>EAGGVFKLIANDGKADRMIMANDLLNDRIKSIMCLRAKQGFSDPTPTLVDIERTHILLINSHYKPFAAMGYEYQKTRPNTGNPTYNSTIQFSIPQFGDFFSDMVVHVQLAATSASAGTVPALPAFIGADDQVLTSTSVVSATENTTSGVYTLYTQSYVNQQGTTQTVAAAATNFVRYCEYPGLRLFKRVKFEVNGNPLDEYTALAAIMYNKFHVPDFKLTGWKRLIGQEVPVEAASNLVNIASTTPWGSPIVALSDVNGTAVTGSPVNA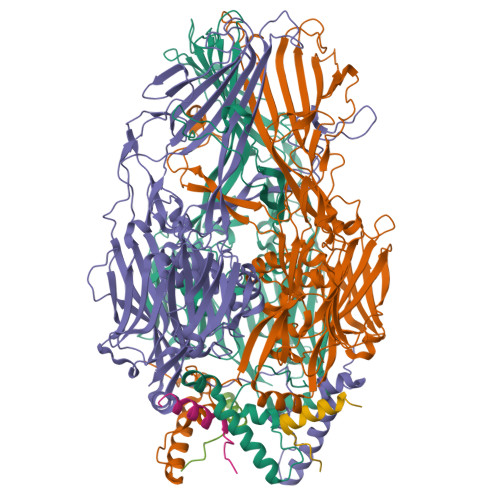AITARKLTQVVFGAQTPKATQEQLNMFVPLLFWFRDPRLAIASVSIPYGQRFITVDIEQQSNILFTAPGNLFLQTTVETLLTTGAGKGTATGVLLTQYNRYTTYTPTLASGSSIDGTQAVQNIELYINNIFVTPEIHDIYIKRIGFTLIRVYREQVQREVNAADQVLQSQLKWPVEFIYLGLRPANNIAAGNTYQWRDWHHLTSVTNEPVYDVSQSYARVSIDDTVAPVGSTTFKQSASQVMQNQYIVPVETETLDTVRVKAHGIELYAQYRAQFYRDYIPWNYGSFNLVTPQDKGALFLNFCLYPGTYQPSGHVNISRAREFYIEYTSSFCDSSNPCDLISIAKCINFLLISDGSAVLRYSTKEFYLQCLILRCI[12x]>[8x]TKVVLGQNQYGKAEVRLVKVTRNTARHEIQDLNVTSQLRGDFEAAHTAGDNAHVVATDTQKNTVYAFARDGFATTEEFLLRLGKHFTEGFDWVTGGRWAAQQFFWDRINDHDHAFSRNKSEVRTAVLEISGSEQAIVAGIEGLTVLKSTGSEFHGFPRDKYTTLQETTDRILATDVSARWRYNTVE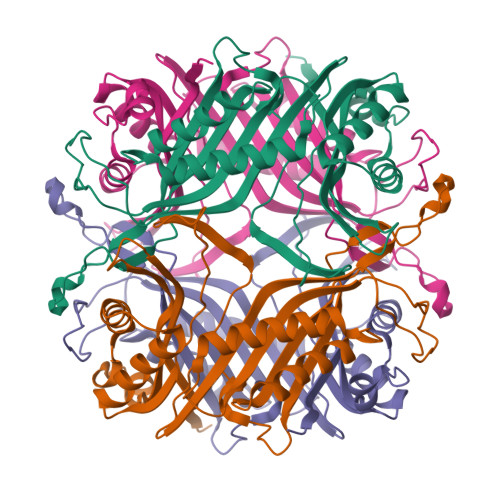VDFDAVYASVRGLLLKAFAETHSLALQQTMYEMGRAVIETHPEIDEIKMSLPNKHHFLVDLQPFGQDNPNEVFYAADRPYGLIEATIQREGSRADHPIWSN>[2x]MTDRDRLRPPLDERSLRDQLIGAGSGWRQLDVVAQTGSTNADLLARAASGADIDGVVLIAEHQTAGRGRHGRGWAATARAQIILSVGVRVVDVPVQAWGWLSLAAGLAVLDSVAPLIAVPPAETGLKWPNDVLARGGKLAGILAEVAQPFVVLGVGLNVTQAPEEVDPDATSLLDLGVAAPDRNRIASRLLRELEARIIQWRNANPQLAADYRARSLTI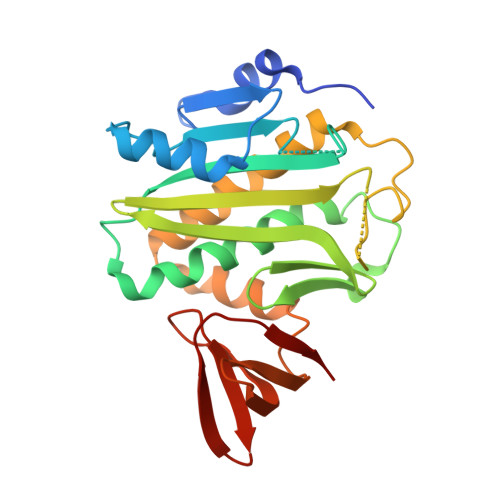GSRVRVELPGGQDVVGIARDIDDQGRLCLDVGGRTVVVSAGDVVHLR> NVSFPASVQLHTAVEMHHWCIPFSVDGQPAPSLRWLFNGSVLNETSFIFTEFLEPAANETVRHGCLRLNQPTHVNNGNYTLLA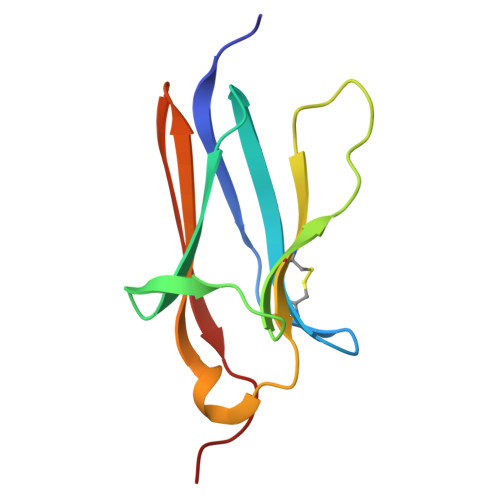ANPFGQASASIMAAFMDNP>[4x]MNLPTAQEVQGLMARYIELVDVGDIEAIVQMYADDATVENPFGQPPIHGREQIAAFYRQGLGGGKVRASLTGPVRASHNGSGAMPFRVEMVW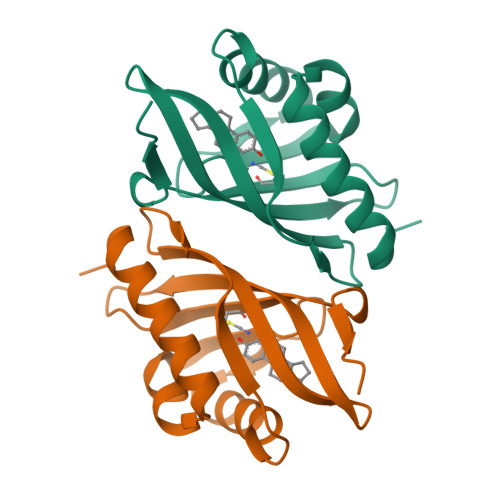NGQPSALDVIDVMRFDEHGRIQTCQAYWSEVNLSVREPQ> GSHMASMSKD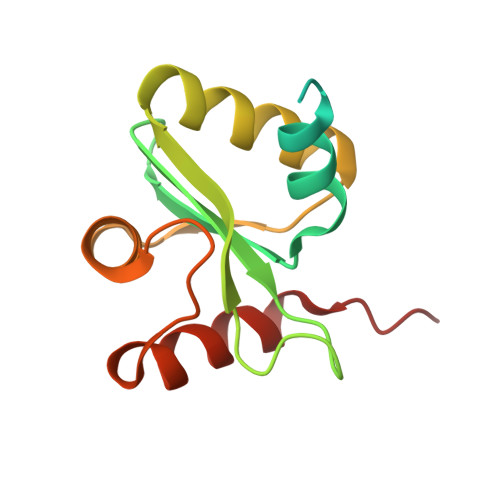EVKREAKDTDGNPEIKGERRRLHSEIQSGSLANNIKKSTVIVKNATHIAICLYYKLGETPLPLVIETGKDAKALQIIKLAELYDIPVIEDIPLARSLYKNIHKGQYITEDFFEPVAQLIRIAIDLDY>[2x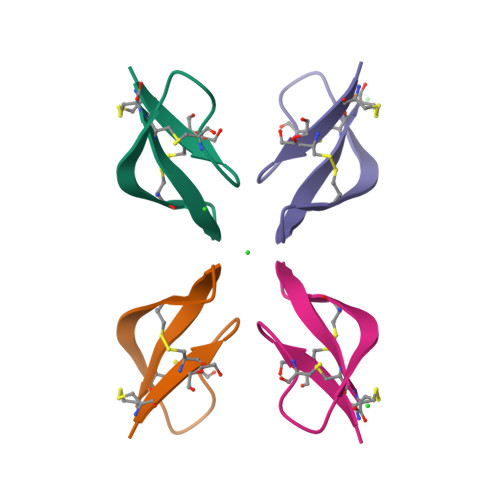]ACYCRIPACIAGERRYGTCIYAGRLWAFCC> VIKELVVSAGESVQITLPKNEVQLNAYVLQEPPKGETYTYD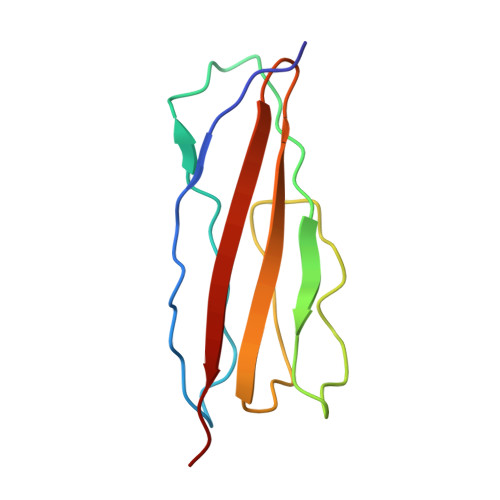WQLITHPRDYSGEMEGKHSQILKLSKLTPGLYEFKVIVEGQNAHGEGYVNVTVKPE>MIELPDAISDGEVRKLVENEFWPEFVRRREKLDRIAQWARGEQPDYLIQNANREKRALLKLAKTPWLGLVVTHFTQALFVDGYRAEGSKENAKGPWQTWNANKMQSKQIAIHRAALTYGYSYARVLPGVALDGANQAEIHGVSPRRLLALYEDQINDEYPKYALELANNGKTVRLYTDTDYYELRMPSPGNFPNEQVIKKVHHGVGVCPFVRYVNMMDLDGFTMGEVEYLVPVASKIDKTDYDRLLAQHYNSWKVKVATGIDDLSEDATPEEQQRAKLILAQDDILMHGNHEAKFYTLPETSLDGFIAAHTQDVEILANNAQVPVWILNGQLANLSADALTAATKGTIQKLYERQVTFGAAHNQVLRLAAHVEGDTEGARDFTASVSWQDTSVRSLAQAVDAYGKAATMLGMPKEFLWGLIPGITKTDVEAMRQHFNDDDEMTQMLLWWTPNGPGGEFAAEIEVDSQTQIIEAQGDVQKDLQDAQAKAQADLAKQNAAAQQRQAVAVAK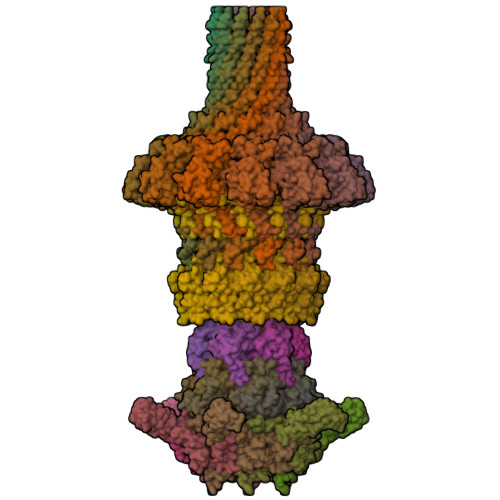ATPAASKAPSTSKAASKRTPKKQGGVSGNDPASRAA[12x];>[6x]MNDETLTVYRGATDNKGNPNKQVHGTVKGVFAWGPGTSTNKFGRDRNFKGESSSLTAELYVKRGADLKARDRIRRANGEEYSVVGHAAWDQGHPFDGFDFGYMVFQVEAVNA;>[6x]MTDFYTIKDAQADLAIAPLNLTVLLAPYSTTPATTLESPTDGSLAIPPGYKSVGHFEKQAGLTLGNEFDSKDIEAYGEPEPIRTIINKRTTTFDFAMYQNQRNVLELIWTQDFSNIQPSEFGGIVLEAPKVPKNIYYRAILVGMDDRNDRPIWLYWLMPKVKLDKLDNQTLNDDNVIEYKPTLKAFRDDVVGYSVAQGFAGPGWRDLVATAGFGEALTALTITPGSPTVTVATGASHTAQLLVEGDNGINYTPDVVFTSSAPDKASVSAAGLVTGVAAGSATITATKGALTATATVTVTA;>MAGLATIDELQTLMSTVFEDDALEQAQLVLDIVSSWARVVSGQMWPDAPANVPDDVRAVVLQASRRELKNPDRVISRQMGPFNVQYSQPPDGFFYPAELAILKRFKRSGGLMTVSTSRGEEGRPWAGKTAYIRYGDGLFPFCSEDEGYGDVVPW[12x];>[6x]MAVVLPDWYEEAFVNVENLFIDMFTDLLPDYESGCWAPDDWLADEIEVKPTIWFFRLPGGRVDWDGRKDECQLQVMVVTGSRDDSWRLMDFVRAMLLPMQGDKYKMADGYTAQIRCAGEVAGPQLLTPGQRIDTRVVTATFKVSVSMKSAKNYKQKLYELWQALRGS> MASWSHPQFEKGASTSLYKKAGLMDSQRSTLVHWFRKGLRLHDNPALSHIFTAANAAPGRYFVRPIFILDPGILDWMQVGANRWRFLQQTLEDLDNQLRKLNSRLFVVRGKPAEVFPRIFKSWRVEMLTFETDIEPYSVTRDAAVQKLAKAEGVRVETHCSHTIYNPELVIAKNLGKAPITYQKFLGIVEQLKVPKVLGVPEKLKNMPTPPKDEVEQKDSAAYDCPTMKQLVKRPEELGPNKFPGGETEALRRMEESLKDEIWVARFEKPNTAPNSLEPSTTVLSPYLKFGCLSARLFNQKLKEIIKRQPKHSQPPVSLIGQLMWREFYYTVAAAEPNFDRMLGNVYCMQIPWQEHPDHLEAWTHGRTGYPFIDAIMRQLRQEGWIHNLARHAVACFLTRGDLWISWEEGQRVFEQLLLDQDWA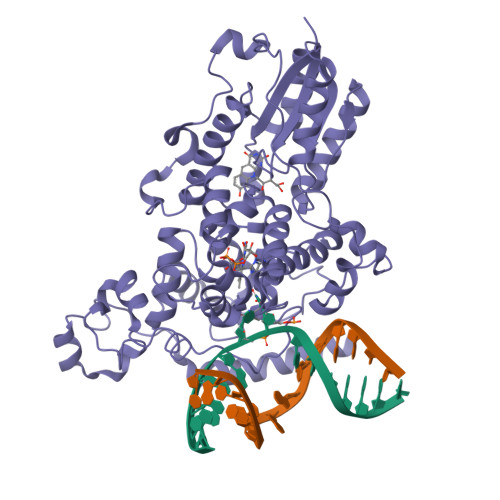LNAGNWMWLSASAFFHQYFRVYSPVAFGKKTDPQGHYIRKYVPELSKYPAGCIYEPWKASLVDQRAYGCVLGTDYPHRIVKHEVVHKENIKRMGAAYKVNREVRTGKEEESSFEEKSET>MSRVPSPPPPAEMSSGPVAESRCYTQIKVVKFSYMWTINNFSFCREEMGEVIKSSTFSSGANDKLKWCLRVNPKGLDEESKDYLSLYLLLVSCPKSEVRAKFKFSILNAKGEETKAMESQRAYRFVQGKDWGFKKFIRRD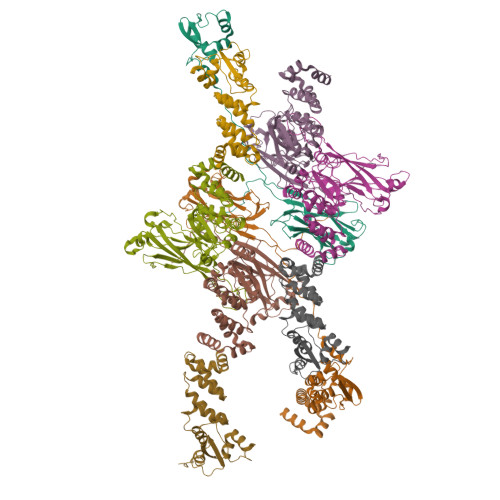FLLDEANGLLPDDKLTLFCEVSVVQDSVNISGQNTMNMVKVPECRLADELGGLWENSRFTDCCLCVAGQEFQAHKAILAARSPVFSAMFEHEMEESKKNRVEINDVEPEVFKEMMCFIYTGKAPNLDKMADDLLAAADKYALERLKVMCEDALCSNLSVENAAEILILADLHSADQLKTQAVDFINYHASDVLETSGWKSMVVSHPHLVAEAYRSLASAQCPFLGPPRKRLKQS[9x]> GAMAAKFRASNIMPSSSFHMSPTSNEDLRKIPDSNPFDATAGYRSLTYEEVLQELVKHKELLRRKDTHIRELEDYIDNL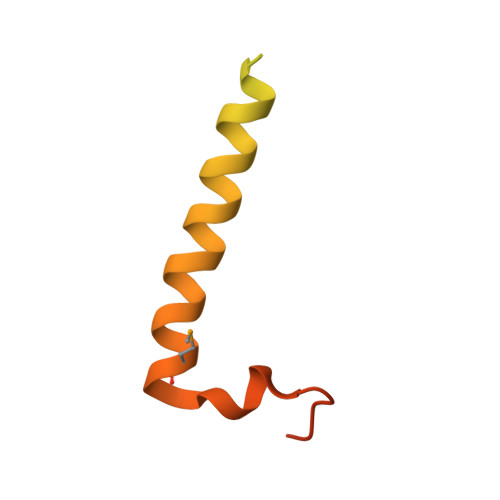LVRVMEETPSILRVPYEPSRKAGKFSNS> KETAAAKFERQHMDSSTSAASSSNYCNQMMKSRNLTKDRCKPVNTFVHESLADVQAVCSQKNV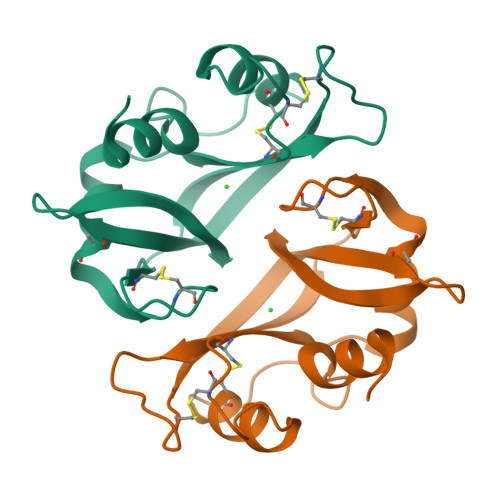ACKNGQTNCYQSYSTMSITDCRETGSSKYPNCAYKTTQANKHIIVACEGNAYVPVHFDASV> STSRGMITDRSGRPLAVSVPVGGGESRRYYPSGEVTAHLIGFTNVDSQGIEGVEKSFDKWLTGQGGGAAHNLALSIDERLQALVYRELNNAVAFNKAESGSAVLVDVNTGEVLAMANSPSYNPNNLSGTPKEAMRNRTITDVFEPGSTVKPMVVMTALQRGVVRENSVLNTIPYRINGHEIKDVARYSELTLTGVLQKSSNVGVSKLALAMPSSALVDTYSRFGLGKATNLGLVGERSGLYPQKQRWSDIERATFSFGYGLMVTPLQLARVYATIGSYGIYRPLSITKVDPPVPGERVFPESIVRTVVHMMESVALPGGGGVKAAIKGYRI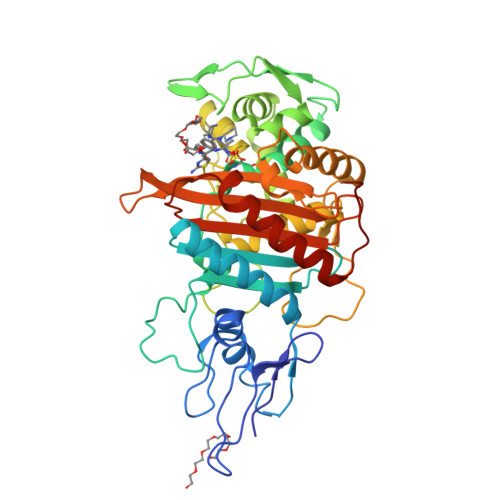AIKTGTAKKVGPDGRYINKYIAYTAGVAPASQPRFALVVVINDPQAGKYYGGAVSAPVFGAIMGGVLRTMNIEPDALTT> EQSSSEIKIVRDEYGMPHIYANDTWHLFYGYGYVVAQDRLFQMEMARRSTQGTVAEVLGKDFVKFDKDIRRNYWPDAIRAQIAALSPEDMSILQGYADGMNAWIDKVNTNPETLLPKQF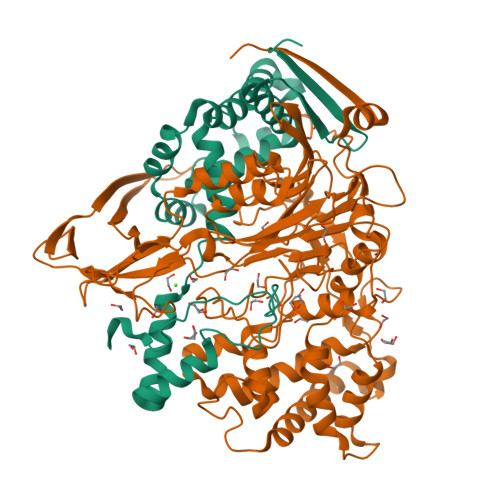NTFGFTPKRWEPFDVAMIFVGTMANRFSDSTSEIDNLALLTALKDKYGVSQGMAVFNQLKWLVNPSAPTTIAVQESNYPLKFNQQNSQTAALLPRYDLPAPMLDRPAKGADGALLALAAGKNRETIAAQFAQGGANGLAGY;> SNMWVIGKSKAQDAKAIMVNGPQFGWYAPAYTYGIGLHGAGYDVTGNTPFAYPGLVFGHNGVISWGSTAGFGDDVDIFAERLSAEKPGYYLHNGKWVKMLSREETITVKNGQAETFTVWRTVHGNILQTDQTTQTAYAKSRAWDGKEVASLLAWTHQMKAKNWQEWTQQAAKQALTINWYYADVNGNIGYVHTGAYPDRQSGHDPRLPVPGTGKWDWKGLLPFEMNPKVYNPQSGYIANWNNSPQKDYPASDLFAFLWGGADRVTEIDRLLEQKPRLTADQAWDVIRQTSRQDLNLRLFLPTLQAATSGLTQSDPRRQLVETLTRWDGINLLNDDGKTWQQPGSAILNVWLTSMLKRTVVAAVPMPFDKWYSASGYETTQDGPTGSLNISVGAKILYEAVQGDKSPIPQAVDLFAGKPQQEVVLAALEDTWETLSKRYGNNVSNWKTPAMALTFRANNFFGVPQAAAEETRHQAEYQNRGTENDMIVFSPTTSDRPVLAWDVVAPGQSGFIAPDGTVDKHYEDQLKMYENFGRKSLWLTKQDVEAHKESQEVLHVQR Ferrous GLB-1 binds O2 with a high affinity and is pentacoordinated in the absence of exogenous heme ligands. The tertiary structure of GLB-1* conforms to the three-over-three α-helical sandwich of the classical globin fold, where the seven/eight helices building up the globin fold are conventionally labelled, A, B..., H, according to their sequential order (topological sites are numbered sequentially within each helix;). The GLB-1* heme distal site resembles that of A. suum Hb, with TyrB10 directly stabilizing the O2 molecule and GlnE7 making a hydrogen bond with the B10 residue. Taken together, the observed functional data suggest for GLB-1 a putative role in vivo related to O2 binding, NO scavenging or O2 storage.

The diffraction data collected at 2.8 Å resolution on GLB-1* crystals grown in the trigonal P3121 space group (two molecules per asymmetric unit) were also refined, yielding Rfactor and Rfree values of 26.9% and 31.9%, respectively, with ideal stereochemical parameters. Superposition of 158 Cα atoms of the two independent molecules, in the trigonal crystal form, yielded a rmsd of 0.53 Å. Comparison of the GLB-1* structures from the tetragonal and trigonal crystal forms yielded rmsd of 0.53 Å and 0.42 Å, for 158 Cα atoms, depending on the chains superposed. The only backbone differences observed in the two crystal forms are located at the N- and C-terminal residues of the polypeptide chain (residues 2 and 159, respectively), and at residues 124-126 of the GH hinge. The crystallographic dimer is identical to the quaternary assembly found in the trigonal crystal form, where two crystallographically independent GLB-1* chains fill the asymmetric unit. The rmsd calculated over the whole dimer in the two crystal forms is 0.50 Å. The dimerization interface observed for the GLB-1 dimer is tightly packed, the stability of the assembly being granted by several hydrophobic interactions, hydrogen bonds (also mediated by water molecules and, in the trigonal crystal form, also by sulphate ions) and salt bridges.

>MSMNRQEISDLCVKSLEGRMVGTEAQNIENGNAFYRYFFTNFPDLRVYFKGAEKYTADDVKKSERFDKQGQRILLACHLLANVYTNEEVFKGYVRETINRHRIYKMDPALWMAFFTVFTGYLESVGSLNDQQKAAWMALGKEFNAESQTHLKNSNLPHV[2x]>SLAEIRTDFNILYSMMKKHEEFRWMRLRI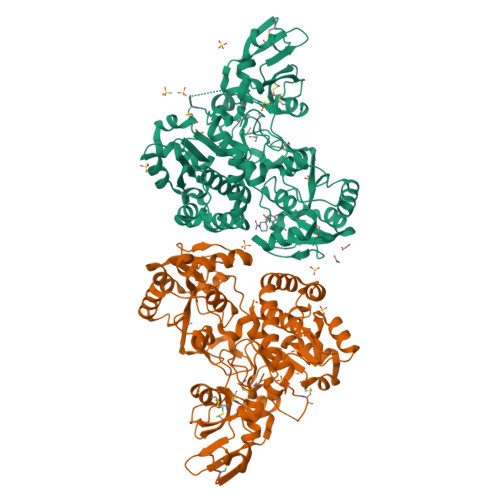RRMADAWIQAIKSLAEKQNLEKRKRKKVLVHLGLLTKESGFKIAETAFSGGPLGELVQWSDLITSLYLLGHDIRISASLAELKEIMGGGGVELIYIDIVGLAQFKKTLGPSWVHYQCMLRVLDSFGTEPEFNHANYAQSKGHKTPWGKWNLNPQQFYTMFPHTPDNSFLGFVVEQHLNSSDIHHINEIKRQNQSLVYGKVDSFWKNKKIYLDIIHTYMEVHATVYGSSTKNIPSYVKNHGILSGRDLQFLLRETKLFVGLGFPYEGPAPLEAIANGCAFLNPKFNPPKSSKNTDFFIGKPTLRELTSQHPYAEVFIGRPHVWTVDLNNQEEVEDAVKAILNQKIEPYMPYEFTCEGMLQRINAFIEKQDFCHGQVMWPPLSALQVKLAEPGQSCKQVCQESQLICEPSFFQHLNKDKDMLKYKVTCQSSELAKDILVPSFDPKNKHCVFQGDLLLFSCAGAHPRHQRVCPCRDFIKGQVALCKDCL[2x]>GPLGSSNLPVRSFSEVCCAEARAAIIQMENNPDETVCNRIWKIHRDLQSSDLTTTVQVMMVYRFISKRVPEGCFAILSGVNTGMYNPRELKRSYVQSLSSGTSC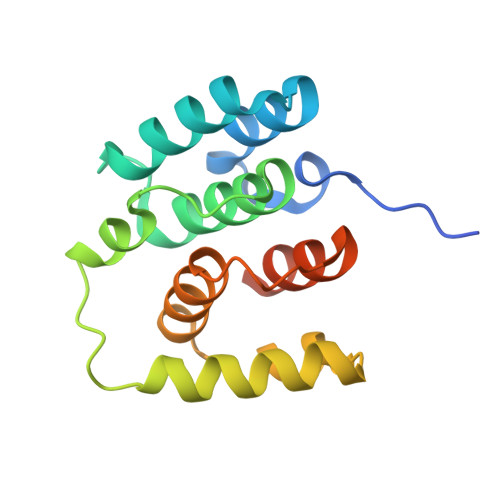EFLRSLDKLAKNLLAVHVCSDVKMSLNKRQVIDFISGEEDPTLHTAEHLT[2x]> MLKIIRAGMYTTVQDGGRHGFRQSGISHCGALDMPALRIANLLVGNDANAPALEITLGQLTVEFETDGWFALTGAGCEARLDDNAVWTGWRLPMKAGQRLTLKRPQHGMRSYLAVAGGIDVPPVMGSCSTDLKVGIGGL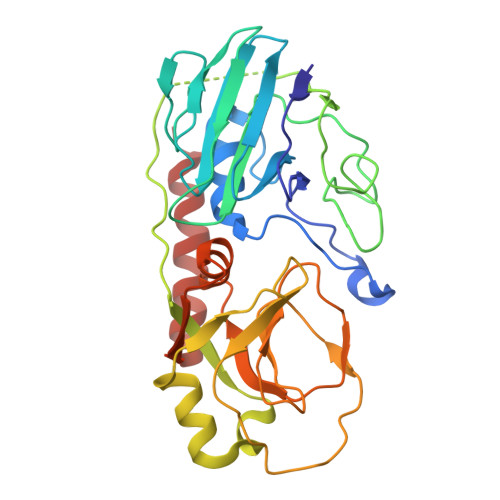EGRLLKDGDRLPIGKSKRDSMEAQGVKQLLWGNRIRALPGPEYHEFDRASQDAFWRSPWQLSSQSNRMGYRLQGQILKRTTDRELLSHGLLPGVVQVPHNGQPIVLMNDAQTTGGYPRIACIIEADMYHLAQIPLGQPIHFVQCSLEEALKARQDQQRYFEQLAWRLHNEN>[2x]GSHMATPPKRSCPSFSASSEGTRIKKISIEGNIAAGKSTFVNILKQLCEDWEVVPEPVARWCNVQSTQDEFEELTMSQKNGGNVLQMMYEKPERWSFTFQTYACLSRIRAQLASLNGKLKDAEKPVLFFERSVYSDRYIFASNLYESECMNETEWTIYQDWHDWMNNQFGQSLELDGIIYLQATPETCLHRIYLRGRNEEQGIPLEYLEKLHYKHESWLLHRTLKTNFDYLQEVPILT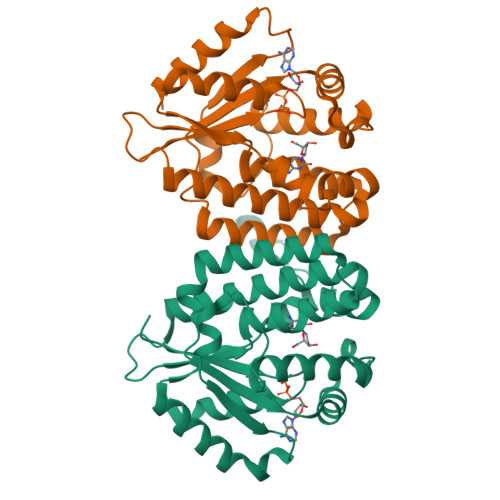LDVNEDFKDKYESLVEKVKEFLSTL> MIKVEIKPSQAQFTTRSGVSRQGKPYSLNEQLCYIDLGNEYPVLVKLTLDEGQPAYAPGLYTVHLSSFKVGQFGSLMIDRLRLVP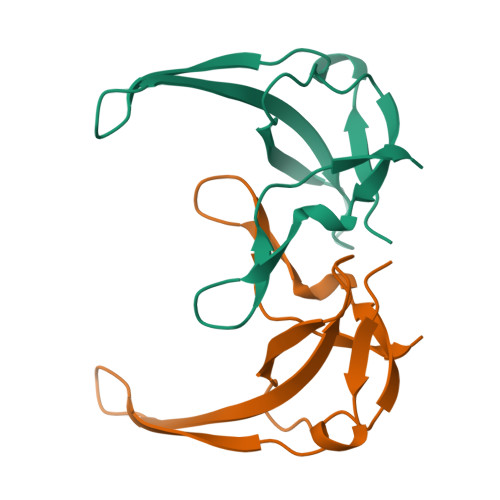AK>[8x]GHAEIMPPPPKPKDRTIPIPISKPPVFIGKDRTEPVKGFHKAMVKTMSAALKIPHFGYCDEVDLTELVKLREELKPIAFARGIKLSFMPFFLKAASLGLLQFPILNASVDENCQNITYKASHNIGIAMDTEQGLIVPNVKNVQIRSIFEIATELNRLQK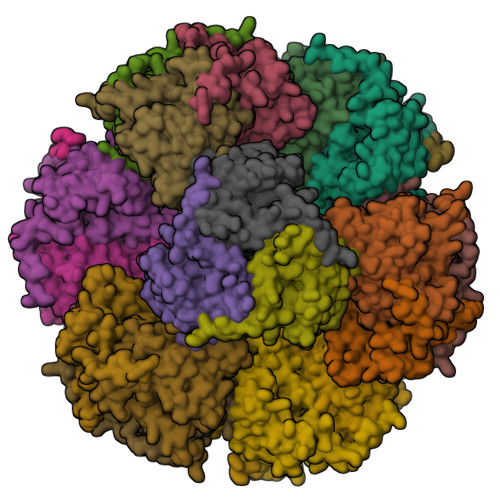LGSAGQLSTNDLIGGTFTLSNIGSIGGTYAKPVILPPEVAIGALGTIKALPRFNEKGEVCKAQIMNVSWSADHRIIDGATVSRFSNLWKSYLENPAFMLLDLK>[2x]FEKAPDSVPETITGGRYSLKDGYYVYLDKQGKQVVGPKNIDNHLQYFDETTGKQVKGDFRSVNGKRIYFNANLGYADDYTTDVAGKLVGYDSNGNQVKAGYVTNSQGKTYYFNNQGEAIIGLKTDNNKTQYFGPDGAQVKGAFQQVNGKNIYFDAQTGYARQNVGFLDGTAKGFDEQGNQIKSGIATDLSGNVYYFDASGKMLTGVQNIDGKKYYFDEQGHRRRNYAGVFNNEFIYFGLDGVGQSAIEYQFEKGLTSQNSVATSHNAAKSYDTKSFTNVDGFLTANSWYRPTDILRNGTKWEPSTETDFRPLLMTWWPDKEVQANYLNYMSALGLGDQKIYTGASSQLDLNNAALIVQEAIEKKISLEKSTKWLDDSIKSFIKSKRKDIQGNLVDTNPGWTIDSETGSTNHLQNGAFIFTNSPLVPEANAAEGNRLINRTPSQQTGNHISYASQPYSGDDWGYELLLGNDVDNSNPIVQAEQLNWIHYLMNFGTITAPQDPDAHLANFDSIRIDAVDNVDADLLQIAGDYFKAAYQVGENDKNANQHIHILQDWSPNDVWYNQQVNGNSQLTMDATMQNQLLASLTRPITSRDSMKSFTKDALLVHRTADNSYNQAVPNYSFIRAHDSEVQTIIAKIISDKHPDLYPTVDKALLAKDSALYDEAFTEYNADMQKISSQKQYTHNNMPSAYAILLTNKDTVPRVYYGDLFTDNGE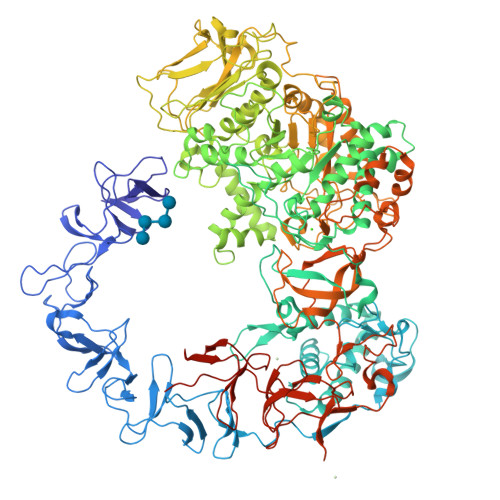YMANKTPYYDAITSLLTARTKFVSGGQSLSVDKNDVLTSVRYGKGALSATDNGSSDTRNQGIGVIVSNNPNLDLNNDKVTLSMGISHAHQAYRPLLLTNSQGIVAYATDSEVPQNLYKTTNDKGELTFDASEIKGYDTVQTSGYLAVWVPVGASDEQDARTIASTEKNNGNSVYHSNAALDSQLIYEGFSNFQTVPSKNASADEYANVIIAKHAADFNKWGVTSFQMAPQYRSSTDGSFLDAVDTVQNGYAFTDRYDLGFNAADGSKNPTKYGTDEDLRNAIKSLHAQKTYDGSSIQVMADFVPDQLYNMPLEQAVSVIRTDKYGVNSENPDIQNIIYAANIKSSGTDYQSIYGGKYLAELQKNPLFKSLFDRIQISTKKTIDPNTRITQWSAKYFNGSNIQGKGINYVLKDWASNKYFNVSSNDDMYSRLPKQLMNQESNTGFIVDDIGVKYYSISGYQAKNTFVEDGNGEWYYFDNDGYMVKSTEESGPLRTVNASSKKYYILPNGVEIRNSFGQDIQGNTYYFDARGEMVTSQYISDDTQNIYYFNNDGTMAKKGGRADPAFLYKVVHHHHHH> GAMASTHHTMKIRSTKFSILNSDHPRIEVKKVFSLSPDVQVTIPYRRFKGKAKVYFQNDQIQGYFSCTDRQIDEIKISAPKNAPLLEPLLDICYYGSFIEPGFEQTFGFYPAGKREFVDSFFMHHSKDHKAFLIHMGLDKDLSLPLSPELNWKEPALSKVCRVTELDS

The three largest gene segments of the Thogotoviruses, THOV, DHOV and JOSV are homologous to those of IAV and code for the heterotrimeric polymerase. In this paper we present the atomic structures of the putative PB2 cap binding and 627 domains of THOV and the putative PA N-terminal endonuclease domains of THOV and DHOV. Despite very low sequence homologies, all domains have similar folds to those of the corresponding IAV polymerase domains. However, the critical active site residues in the putative cap binding and endonuclease domains are not conserved in THOV and DHOV and, contrary to the case of IAV polymerase, neither domain shows the expected in vitro biochemical activity.

Sequence alignments were used to define a putative cap-binding domain in THOV PB2 subunit, even though the sequence identity of this region of PB2 compared to IAV PB2 is only about 8%. A construct comprising residues 323–486 could be expressed, crystallised in two different forms, and its structure determined at 1.8 Å resolution. Once again, the low sequence homology with the corresponding IAV domain necessitated de novo structure solution by selenium SAD, rather than by molecular replacement. Despite the low sequence identity the THOV domain is clearly structurally homologous to that of IAV as indicated by the close correspondence of secondary structure elements shown in the structure based alignment. Firstly, the so called ‘348-loop’ formed by the β3–β4 hairpin is longer in THOV and its extremity orientates away from the body of the domain towards the solvent, whereas in IAV the tip packs against bends the body of the molecule. Secondly, the prominent, solvent exposed ‘424-loop’ of the IAV cap-binding domain is absent due to truncation in THOV. Whereas in THOV, Tyr413 is similarly placed to Phe404, there is no equivalent of His 357 for the other side of the aromatic sandwich. Furthermore, there are no polar residues in THOV that could specifically hydrogen bond to the guanosine base, since Glu361 and Lys376 in IAV are non-conservatively replaced by respectively Ala370 and Cys385 (Tyr and Gly in DHOV). Finally, in all three crystallographically independent examples of the THOV domain, the equivalent position of the m7G itself is occupied by the side-chain of Arg344, with its guanidinium group stacking with the side-chain and making two hydrogen bonds to the main-chain carbonyl oxygen of Tyr413. The THOV domain is not retained by m7G Sepharose under conditions where IAV cap-binding domain is and, similarly, no binding of m7GTP could be detected by isothermal calorimetry experiments under conditions where IAV cap-binding domain shows clear binding with a Kd of 2.7 µM.> MQLSKEPRELNREWLIVLSELGQGAFGIVYEASLSEPKAPEIQVAAKSLRKDAMDNEREE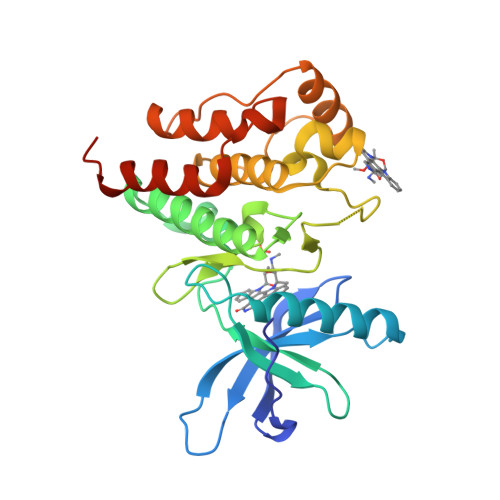LLEEALVMAQMEHANVVGLIGVITKGRPIYVVLEHMRNGSLKDYVMNKTCTPAQQVTWSRQVASGMAHIHSLGFIHRDLAARNVLLSASLTAKVADFGLARESTDDAYYRSRGGNVPVRWTAPEALEDNIFSEKSDVWAFGVLMYEVYTKAAMPYTGWNNQRVWIEVTNGFRLPCPADCPLPVFKIMSMCWLHDRHERPSFETLVKALAALETDSDMSSLFQS> MERYENLFAQLNDRREGAFVPFVTLGDPGIEQSLKIIDTLIDAGADALELGVPFSDPLADGPTIQNANLRAFAAGVTPAQCFEMLALIREKHPTIPIGLLMYANLVFNNGIDAFYARCEQVGVDSVLVADVPVEESAPFRQAALRHNIAPIFICPPNADDDLLRQVASYGRGYTYLLSRSGVTGAENRGALPLHHLIEKLKEYHAAPALQGFGISSPEQVSAAVRAGAAGAISGSAIVKIIEKNLASPKQMLAELRSFVSAMKAASRA;> MTTLLNPYFGEFGGMYVPQILMPALNQLEEAFVRAQ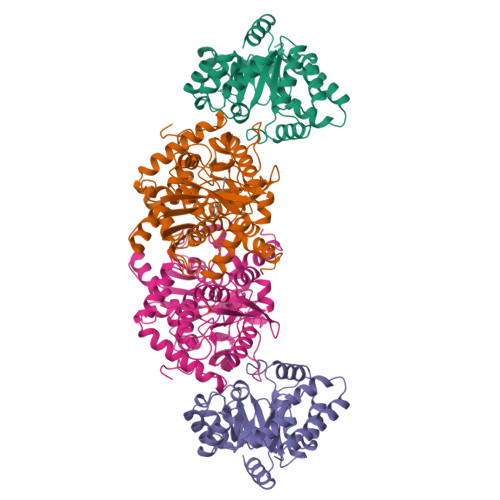KDPEFQAQFADLLKNYAGRPTALTKCQNITAGTRTTLYLKREDLLHGGAHTTNQVLGQALLAKRMGKSEIIAETGAGQHGVASALASALLGLKCRIYMGAKDVERQSPNVFRMRLMGAEVIPVHSGSATLKDACNEALRDWSGSYETAHYMLGTAAGPHPYPTIVREFQRMIGEETKAQILDKEGRLPDAVIACVGGGSNAIGMFADFINDTSVGLIGVEPGGHGIETGEHGAPLKHGRVGIYFGMKAPMMQTADGQIEESYSISAGLDFPSVGPQHAYLNSIGRADYVSITDDEALEAFKTLCRHEGIIPALESSHALAHALKMMREQPEKEQLLVVNLSGRGDKDIFTVHDILKARGEI>MALNSINTNAGAMIALQNLNGTNSELTTVQQRINTGKKIASAKDNGAIWATAKNQSATAASMNAVKDSLQRGQSTIDVALAAGDTITDLLGKMKEKALAASDCSLNTASFNALKSDFD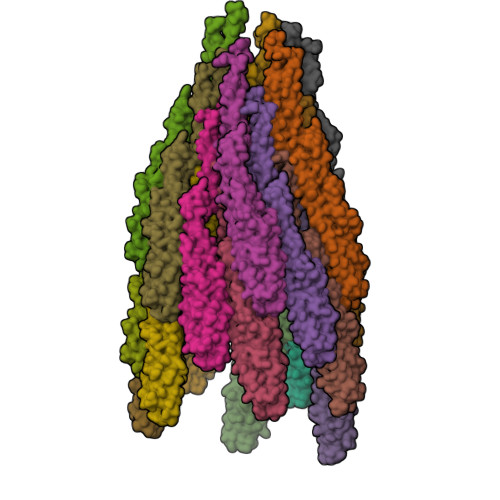SLRDQIEKAATSAKFNGVSIADGSTTKLTFLANSDGSGFTVNAKTISLAGIGLTTTSTFTTAAAAKTMIGTIDTALQTATNKLASLGTSSVGLDTHLTFVGKLQDSLDAGVGNLVDADLAKESAKLQSLQTKQQLGVQALSIANQSSSSILSLFR[20x]>[2x]CAAAGAAAAG;>CTXTCTTTG[2x]

With this in mind we describe reduced-charge oligonucleotides containing artificial LNA-amide linkages with improved gymnotic cell uptake, RNA affinity, stability and potency. We solved several X-ray structures to determine the effects of LNA and amide modifications on duplex structure and conformation. These are the first crystal structures of DNA:RNA hybrids that contain amide linkages. The sequence of the modified DNA:RNA hybrid duplexes was based on the corresponding unmodified version (d-CTTTTCTTTG/rCAAAGAAAAG)51 (the location of the amide is underlined).

Good quality crystals diffracting between 2.5–2.8 Å resolution were obtained for the DNA:RNA hybrid in which the DNA strand contains an amide linkage flanked by DNA on both sides, LNA on both sides and with LNA only on the 5′-side. The hybrids with amide and LNA-amide backbones are structurally very similar to the unmodified duplex (all-atom RMSD 0.4 Å) as shown by their superimposition. All structures adopt the A-conformation with sugar puckers clustering around C3′-endo. Between each structure, the orientation of the backbone is consistent, directing the amide oxygen into the major groove. Other atomic positions of the backbones also show close similarity, and the presence of 3′-LNA causes no significant distortion. 5′-LNA does however cause some structural displacement; the 5′-sugars in the LNA-amide-DNA and LNA-amide-LNA structures are shifted slightly outwards compared to the DNA-amide-DNA and unmodified strands. Despite this, the positioning of the amide backbone remains consistent between each structure. In summary, combined LNA and amide modifications have minimal effect on the duplex structure, and are excellent mimics of natural phosphodiesters. Importantly, ON4LNA-Am-LNA, in which the amide is surrounded by LNA sugars, gave the greatest increase in stability (+5.1 ˚C).2,10,23-TRIMETHYL-TETRACOSANE | C27 H56 | 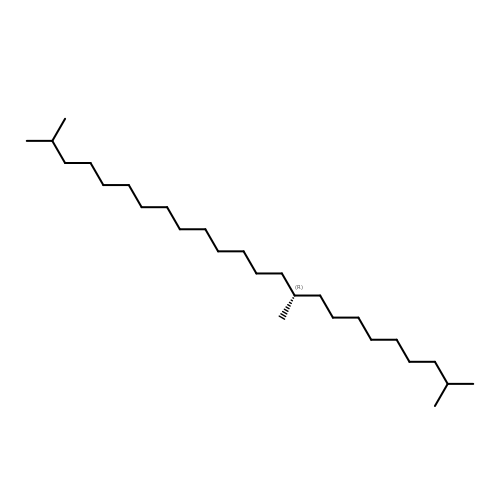ZADHKSJXSZBQFB-HHHXNRCGSA-N>MDIGINSDPHHHHHHGGLDIVNNATGDDNRDDLNIRTYGATETSSLIMLRARGTASAPAAVQTGDRLGGVLFRGWNGTAWMGSGQILSVAEENFTTAVKTNLQFHVGGAGEAMRISNTGNVGIGTTTTTEKLNVQGNVAVSGEITSVRSWGIKRGPTSFSANYINVWNSGYHVGSSIDCTTSTTGCRILKAGTYEIRCVQRAGTSGNSVYVGIALNGDRTALESRNDVLWNHSHTAYSGSYTESNFMGTLSANDLITCGAPVNTMAADLVYAVPAYNGTMQIKRVD[3x]

Bdellovibrio bacteriovorus is a bacterium that preys upon a wide range of other Gram-negative bacteria, entering their periplasm and consuming them from within. Proteomic and structural analyses of vesicle contents reveal several fibre-like proteins, which we name the mosaic adhesive trimer (MAT) superfamily, and show localization on the predator surface before prey encounter. Structural studies reveal a variety of domain usages (and therefore binding capabilities) at the fibre C-termini, placing these on intertwined trimeric β-prisms. Using independent but complementary approaches, we identified and characterized a MAT superfamily of trimeric fibre proteins with diverse adhesive tips, able to fulfil the long-sought-after role of multiplicity of molecular recognition and handling of diverse epitopes (across a wide prey range), by the bacterial predator B. bacteriovorus.

We next characterized two more divergent NS74s, Bd2439 and Bd2734, obtaining a tip-only variant of Bd2734 (residues T691–L843, 1.8 Å) and a longer construct of Bd2439 (G837–D1107, 1.6 Å). The resulting structures reveal that both proteins use a related fold. Bd2439 is modular, formed by a β-helix N850–V968, a R969 linker that coordinates the carboxy terminus and a compact β-domain tip from S970–D1107. Mapping a sequence alignment to Bd2439 identifies a conserved interfacial pocket (Y1031, R1040, E1044, H1053 and H1055 from one monomer; R1022 and Y1097 from another). These residues coordinate two hydroxyl groups from a bound ethylene glycol. Bd2439 showed strong binding to Proteus mirabilis OXK glycan, with weaker (but significant) binding to glycans from E. coli K-235 and Serratia marcescens. The multiplicity of the MAT family prevents exhaustive and absolute specificity determination (as suggested by our knockout phenotypes), but we use Bd2439 as a proof of principle to link to recognition of bacteria with Proteus-like O-antigen chemistries, revealing a molecular basis for B. bacteriovorus prey handling.> MGQTATTVPEFPSKLDWLNTAPLQFRRDLKGKVVILDFWTYCCINCMHVLPDLEFLEKKYKDMPFTVVGVHSAKFDNEKDLDAIRNAVLRYDISHPVVNDGDMYMWRELGINSWPTFAVVSPNGKVIAQIAGEGHRKDLDDVVAAALTYYGGKNVLDSTPLPTRLEKDNDPRLATSPLKFPGKLAIDTLNNRLFISDSNHNRIIVTDLEGNFIVQIGSSGEEGFQDGSFEDAAFNRPQGLAYNAKKNLLYVADTENHALREIDFVNERVQTLAGNGTKGSDYQGGRKGTKQLLNSPWDVCFEPVNEKVYIAMAGQHQIWEYSVLDGITRVFSGNGYERNLNGSTPQTTSFAQPSGISLGPDLKEAYIADSESSSIRALDLQTGGSR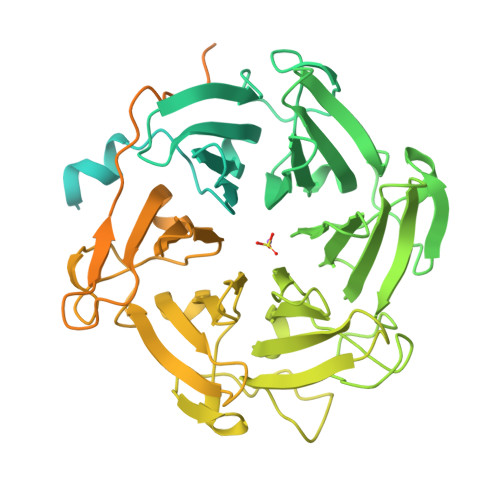LLAGGDPYFSENLFKFGDNDGVGAEVLLQHPLGVLCANDGQIYLTDSYNHKIKKLDPVTKRVVTLAGTGKAGFKDGKVKGAQLSEPAGLAITENGRLFVADTNNSLIRYIDLNKGEDSEILTLELKGVQPPTPKAKSLKRLRKRASADTKIVKVDSVTSREGDLNLKISLPDGYHFSKEARSKFVVDVEPENAVAIDPTEGTLSPEGSTMLHFIQSSTSASVGKISCKVYYCKEDEVCLYQSVQFEVPFKVESELSASPTITFTVTPRAPDAGGLQLQGTR>[2x]MSKQPMTPFEAIGGEQCIEILVDTFYSYVSK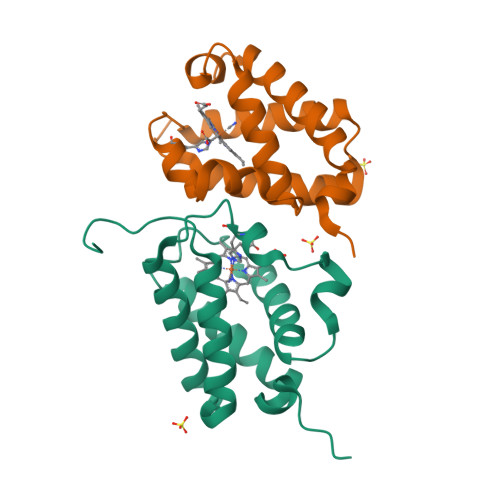HPDLSPIFPDDLTETARKQKQFLTQYLGGPNLYTEEHGHPMLRARHLPFEITPKRAEALLSCMEQAMDDTGVHGHIREFVFERLALTAQHMVNTPNETGEI> MEQLRGLYPPLAAYDSGWLDTGDGHRIYWELSGNPNGKPAVFIHGGPGGGISPHHRQLFDPERYKVLLFDQRGCGRSRPHASLDNNTTWHLVADIERLREMAGVEQWLVFGGSWGSTLALAYAQTHPERVSEMVLRGIFTLRKQRLHWYYQDGASRFFPEKWERVLSILSDDERKDVIAAYRQRLTSADPQVQLEAAKLW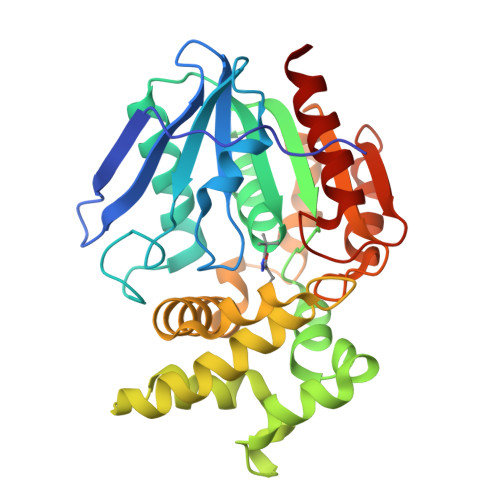SVWEGETVTLLPSRESASFGEDDFALAFARIENHYFTHLGFLESDDQLLRNVPLIRHIPAVIVHGRYDMACQVQNAWDLAKAWPEAELHIVEGAGHSYDEPGILHQLMIATDRFAGK4-amino-N-[(1R,3S)-3-hydroxycyclopentyl]-1,2,5-oxadiazole-3-carboxamide | C8 H12 N4 O3 | 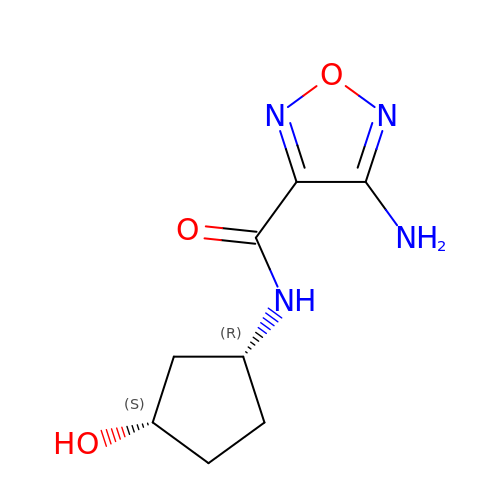UDKGUOUTPCVPOO-UHNVWZDZSA-N>GSPAKIKIVAPLESALIPGGETYQLRCDIMSTPAATIHWKFNGKLIQGSNELNVEEKLLNFGKAIVDTGIVASILTIQCPSAENSGTYSCVGYNGHQTIETVAEVEIEGEASGCRSNHKSAPEIVFWTDSRFEMTGNVATLVCRANQQVDWVWMSNDELVKNNDKFTVLSNGDLVIKNIVWDDMGTYTCIARNQFGEARQETFLYPTAHHHHHH[4x];>VPAPGETRACGRKLISLVMAVC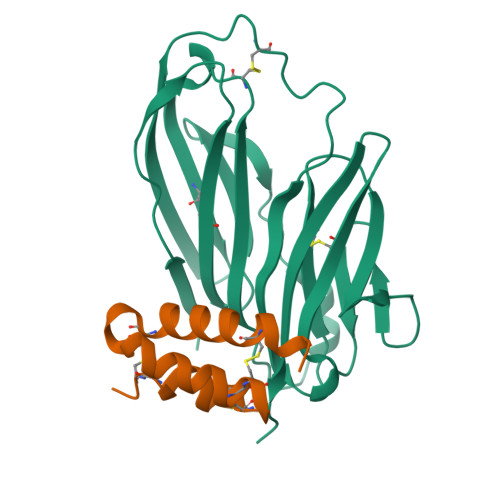GDLCNPQEGKDIATECCGNQCSDDYIRSACCPHHHHHH[4x]Almost all prokaryotic genomes encode toxin–antitoxin (TA) systems. These loci consist of bicistronic operons that encode for a bacterial toxin and its cognate inhibitor, which neutralizes the toxin under dormant conditions. The epsilon/zeta and the PezAT system form similar heterotetrameric complexes in which two antitoxin molecules inhibit two toxins. In conclusion, we have demonstrated that zeta and PezT toxins are UNAG kinases that form UDP-N-acetylglucosamine-3′-phosphate (UNAG-3P) from UNAG using ATP and Mg2+ as a cofactor. We further showed that the formation of UNAG-3P yields a potent inhibitor of the enzyme MurA, which synthesizes the first committed step of bacterial cell wall synthesis.

Once bound to the antitoxin, side chain groups of the antitoxin block the ATP binding site. The second substrate binding site, however, remains unaffected by the antitoxin. Thus, we surmised that PezT and zeta toxins are still able to bind UNAG even if they are inhibited by the antitoxin. Indeed, we could determine the crystal structure of the epsilon/zeta TA complex from S. pyogenes bound to UNAG at 2.7 Å resolution. UNAG binds to a deep cleft at the molecular surface of the zeta toxin. The side chain group of Asp67 forms a hydrogen bond (3.2 Å) to the 3′-hydroxyl group of the amino sugar moiety of UNAG. Based on superposition with structurally related phosphotransferases, this particular side chain of the zeta toxin had been suggested to be the catalytic base, which deprotonates the substrate. Thr118 of the zeta toxin formed a hydrogen bond with an oxygen atom of the β-phosphate group of UNAG (2.8 Å), and exchange of this conserved residue in the PezT toxin to a valine residue also yielded a nontoxic variant. Additional specific contacts between the zeta toxin and UNAG are electrostatic interactions of Arg120 with the phosphate groups of UDP. Apart from van der Waals interactions, specific hydrogen bonds are formed between Thr128 and the uracil base and between Glu100 and the 2′-hydroxyl group of the UDP ribose.

>MAVTYEKTFEIEIINELSASVYNRVLNYVLNHELNKNDSQLLEVNLLNQLKLAKRVNLFDYSLEELQAVHEYWRSMNRYSKQVLNKEKVA[2x];>MANIVNFTDKQFENRLNDNLEELIQGKKAVESPTAFLLGGQPGSGKTSLRSAIFEETQGNVIVIDNDTFKQQHPNFDELVKLYEKDVVKHVTPYSNRMTEAIISRLSDQGYNLVIEGTGRTTDVPIQTATMLQAKGYETKMYVMAVPKINSYLGTIERYETMYADDPMTARATPKQAHDIVVKNLPTNLETLHKTGLFSDIRLYNREGVKLYSSLETPSISPKETLEKELNRKVSGKEIQPTLERIEQKMVLNKHQETPEFKAIQQKLESLQPPTPPIPKTPKLPGI[2x]> MALSRGLPRELAEAVAGGRVLVVGAGGIGCELLKNLVLTGFSHIDLIDLDTIDVSNLNRQFLFQKKHVGRSKAQVAKESVLQFYPKANIVAYHDSIMNPDYNVEFFRQFILVMNALDNRAARNHVNRMCLAADVPLIESGTAGYLGQVTTIKKGVTECYECHPKPTQRTFPGCTIRNTPSEPIHCIVWAKYLFNQLFGEEDADQEVSPDRADPEAAWEPTEAEARARASNEDGDIKRISTKEWAKSTGYDPVKLFTKLFKDDIRYLLTMDKLWRKRKPPVPLDWAEVQSQGEETNASDQQNEPQLGLKDQQVLDVKSYARLFSKSIETLRVHLAEKGDGAELIWDKDDPSAMDFVTSAANLRMHIFSMNMKSRFDIKSMAGNIIPAIATTNAVIAGLIVLEGLKILSGKIDQCRTIFLNKQPNPR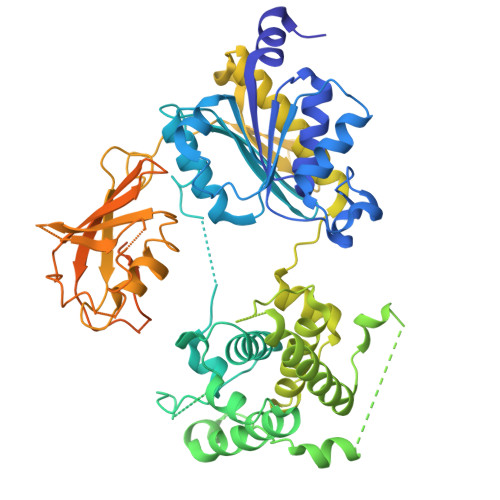KKLLVPCALDPPNPNCYVCASKPEVTVRLNVHKVTVLTLQDKIVKEKFAMVAPDVQIEDGKGTILISSEEGETEANNHKKLSEFGIRNGSRLQADDFLQDYTLLINILHSEDLGKDVEFEVVGDAPEKVGPKQAEDAAKSITNGSDDGAQPSTSTAQEQDDVLIVDSDEEDSSNNADVSEEERSRKRKLDEKENLSAKRSRIEQKEELDDVIALD alpha-D-quinovopyranose 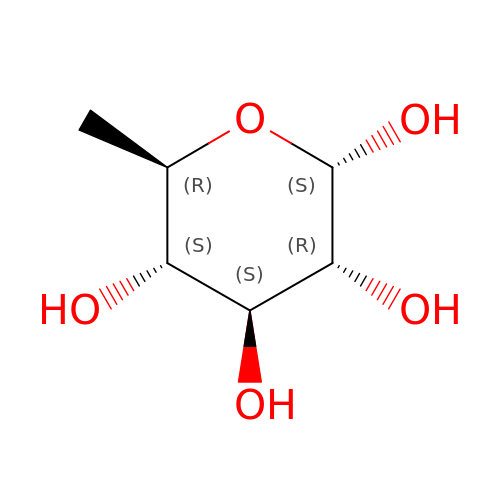| C6 H12 O5 | SHZGCJCMOBCMKK-DVKNGEFBSA-N> MLGSGFKAERLRVNLRLVINRLKLLE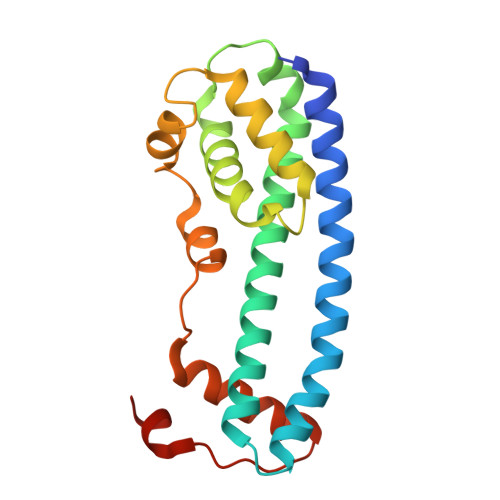KKKTELAQKARKEIADYLAAGKDERARIRVEHIIREDYLVEAMEILELYCDLLLARFGLIQSMKELDSGLAESVSTLIWAAPRLQSEVAELKIVADQLCAKYSKEYGKLCRTNQIGTVNDRLMHKLSVEAPPKILVERYLIEIAKNYNVPYEPDSVVMAEAPP>MGSDKIHHHHHHERNKTLYWGGALWSPPSNWNPFTPWNAVAGTIGLVYEPLFLYDPLNDKFEPWLAEKGEWVSNNEYVLTLRKGLRWQDGVPLTADDVVFTFEIAKKYTGISYSPVWNWLGRIERVDERTLKFVFSDPRYQEWKQMLINTPIVPKHIWENKTEEEVLQAANENPVGSGPYYVESWADDRCVFKKNGNWWGIRELGYDPKPERIVELRVLSNNVAVGMLMKGELDWSNFFLPGVPVLKKAYGIVTWYENAPYMLPANTAGIYINVNKYPLS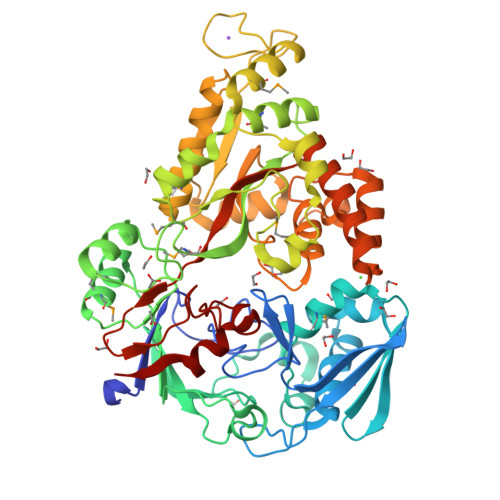IPEFRRAMAYAINPEKIVTRAYENMVTAANPAGILPLPGYMKYYPKEVVDKYGFKYDPEMAKKILDELGFKDVNKDGFREDPNGKPFKLTIECPYGWTDWMVSIQSIAEDLVKVGINVEPKYPDYSKYADDLYGGKFDLILNNFTTGVSATIWSYFNGVFYPDAVESEYSYSGNFGKYANPEVETLLDELNRSNDDAKIKEVVAKLSEILLKDLPFIPLWYNGAWFQASEAVWTNWPTEKNPYAVPIGWNGWWQLTGIKTLFGIEAK[2x]1-(beta-D-glucopyranosyl)-5-(pent-1-yn-1-yl)pyrimidine-2,4(1H,3H)-dione | C15 H20 N2 O7 | 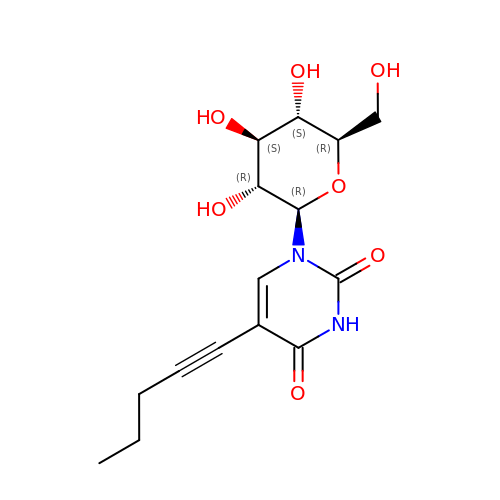XHEMRIMZCOFGEX-YGEZULPYSA-N[({[4-(1H-tetrazol-5-yl)-2-(trifluoromethyl)phenyl]sulfonyl}amino)methyl]boronic 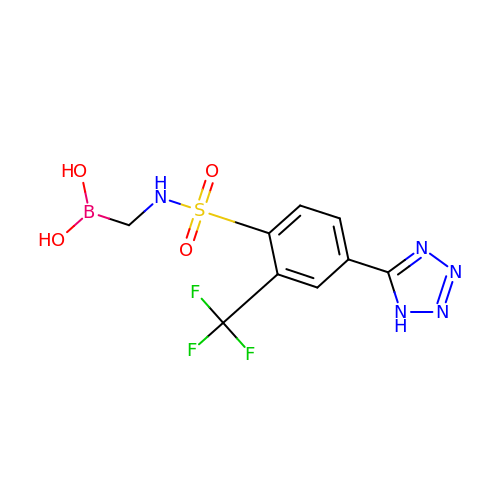acid | C9 H9 B F3 N5 O4 S | KJEUORQIESDSSV-UHFFFAOYSA-N> SDTAPAGFQLERVVILSRHGVRAPTKMTQTMRDVTPHQWPEWPVKLGYITPRGEHLISLMGGFYRERFQQQGLLPKDNCPTPDAVYVWADVDQRTRKTGEAFLAGLAPQCDLAIHHQQNTQQADPLFHPVKAGICSMDKSQVHAAVEKQAGTPIETLNQRYQASLALMSSVLDFPKSPYCQQHNISKLCDFSQAMPSRLAINDDGNKVALEGAVGLASTLAEIFLLEHAQGMPKVAWGNIHTEQQWNSLLKLHNAQFDLMSRTPYIAKHNGTPLLQTIAHALGSNITSRPLPDISPDNKILFIAGHDTNIANISGMLGMTWTLPGQPDNTPPGGALVFERWVDNAGKPYVSVNMVYQTLAQLHDQAPLTLQHPAGSVRLNIPGCSDQTPDGYCPLSTFSRLVSHSVEPACQLP

Phytases (myo-inositol hexakisphosphate phosphohydrolases) catalyse the hydrolysis of phytate into inorganic phosphate (Pi) and lower phosphorylated myo-inositols. Here we report the identification of two HAPPs from the enterobacteria Hafnia alvei (HaPhy) and Yersinia kristensenii (YkPhy), together with biochemical studies of their pH and temperature optima, as well as their phytate degradation pattern, which show that they are 6-phytases. The enzymes share a common catalytic site architecture located at the interface of the two domains involving the conserved N-terminal active site motif RHGXRXP and the C-terminal HD. The two-step reaction involves a nucleophilic attack on the phosphorous by the histidine from the RHGXRXP motif to form a covalent phosphohistidine intermediate while the aspartic acid of the HD motif serves as a proton donor to the oxygen atom of the scissile phosphomonoester bond.

The apoHaPhy structure at pH 7.5 was refined at a resolution of 1.90 Å with one monomer in the asymmetric unit. The first two residues of the N-terminus, five residues (184–188) in a small disordered loop and three residues (414–416) at the C-terminus were disordered. Six side chains on the surface were modelled as dual conformers, while Glu181, Gln182 and His183 have poorly defined side chains and lie at the start of the disordered loop. The model includes seven glycerol, five acetate and 306 water molecules. The overall fold conforms to that of known HAPs with an α domain (residues 25–45 and 137–264) and a α/β domain (the remaining residues) with two α helices on each side of a twisted β-sheet. The two central helices of the α domain form part of the active site, which lies in a pocket at the interface of the two domains. HaPhy possesses four disulphide bridges involving cysteines 79/110, 135/410, 180/189, and 384/393, the latter being highly conserved in all known HAP structures. While Arg20 in EcPhy moves significantly to form a contact with the scissile phosphate, in HaPhy the corresponding Arg22 is already in the “contact-ready” conformation in the apo-structure, superimposing very well on the ligand-bound arginines from both the EcPhy and HaPhy complexes. Yet another difference from the EcPhy active site structure is that there is no change in the conformation of Glu222 (Glu219 in EcPhy) between the apo and ligand-bound states.>PAPVEVTYKNMRFLITHNPTNATLNKFIEELKKYGVTTIVRVCEATYDTTLVEKEGIHVLDWPFDDGAPPSNQIVDDWLSLVKIKFREEPGCCIAVHCVAGLGRAPVLVALALIEGGMKYEDAVQFIRQK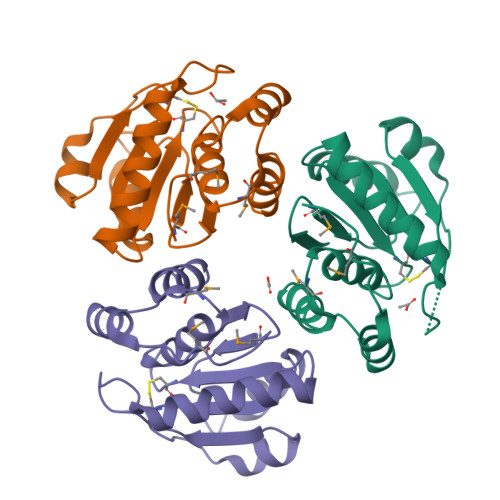RRGAFNSKQLLYLEKYRPKMRLRF[3x]>HHHHHHENLYFQGMAVSPSPLRIFTAGGTIDKDFRLEENGLVVGDPFVAEVLKTARLAGAVSIVALSRKDSLDFTEADREAIGRAVGQAVEDHILLTHGTDTMVETARYLGGLPELAGKTVVLSGAMVPGRVGGSDAAFNIGFACAAALMLAPGVYIAMHGKVFDPAKTRKNRGLGRFEPIDDQE[8x]

L‐Asparaginases (ASNases) catalyze the hydrolysis of L‐Asn to L‐Asp and ammonia. In contrast, the chain of ASNase from Rhodospirillum rubrum, reported here and referred to as RrA, consists of only 172 amino acid residues. RrA is homologous to the N‐terminal domain of typical bacterial class 1 ASNases and exhibits millimolar affinity for L‐Asn. Crystal structures of the wild‐type RrA, both with and without bound L‐Asp, as well as structures of several RrA mutants, reveal topologically unique tetramers.

Based on the previously published results for typical class 1 ASNases (Derst et al., 1994; Schalk et al., 2016), we tested two mutants, RrA(Y21A) and RrA(Y21F). Finally, the Y21F variant grown in the absence of L‐Asp crystallized in space group C2 with two complete tetramers in the a. u. RrA(Y21F), also grown without added L‐Asp, nonetheless contained L‐Asp in the active sites of some protomers, presumably co‐purified from the cell lysate. Other protomers contained water molecules, ethylene glycol, and/or chloride ions, all contributed by the buffer. In all protomers without a bound L‐Asp we observed a putative H‐bond between Thr16 and OD1 of Asn26, which belongs to the same chain as Phe21. The distance between Thr16(OG1) and Lys19(NZ) was longer than in RrA(wt), exceeding 4 Å in all eight molecules. Although both were less active than RrA(wt), RrA(Y21F) is somewhat more active than RrA(Y21A), which is opposite to the results obtained for typical class 1 ASNases. While it is quite plausible that in RrA Tyr21 contributes to proton transfer from the primary nucleophile (Thr16), almost certainly its side chain also contributes to stabilization of the tetramer. In this role, substituting Tyr with Phe preserves this role better than the mutation Tyr → Ala.S-{2-[(2-chloro-4-sulfamoylphenyl)amino]-2-oxoethyl} 6-methyl-3,4-dihydroquinoline-1(2H)-carbothioate | C19 H20 Cl N3 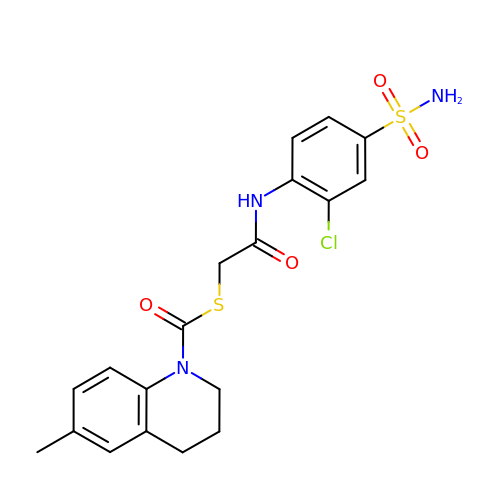O4 S2 | AWAKIULNKVOBKE-UHFFFAOYSA-N>MEPFRNIGIIGRLGSTQVLDTIRRLKKFLIDRHLHVILEDTIAEVLPGHGLQTCSRKIMGEICDLVVVVGGDGSMLGAARALARHKVPVLGINRGSLGFLTDIRPDELEAKVGEVLDGQYIVESRFLLDAQVRRGIDSMGQGDALNDVVLHPGKSTRMIEFELYIDGQFVCSQKADGLIVATPTGSTAYALSAGGPIMHPKLDAIVIVPMYPHMLSSRPIVVDGNSELKIVVSPNMQIYPQVSCDGQNHFTCAPGDTVTISKKPQKLRLI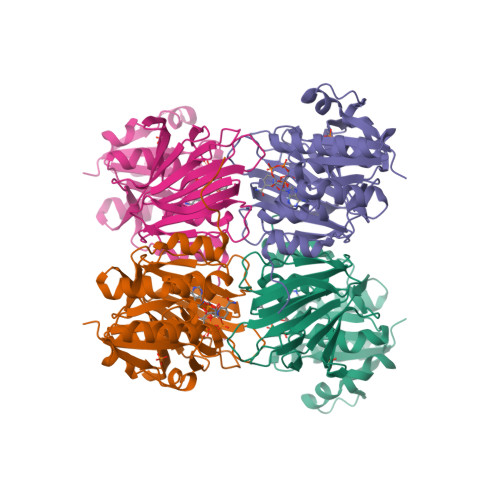HPIDHNYYEICRTKLGWGSRLGGGDLEHHHHHH[2x]>MSLTNKKNLRVVALAPTGRYFASIISSLEILETAAEFAEFQGFMTHVVTPNNRPLIGRGGISVQPTAQWQSFDFTNILIIGSIGDPLESLDKIDPALFDWIRELHLKGSKIVAIDTGIFVVAKAGLLQQNKAVMHSYFAHLFGELFPEIMLMTEQKALIDG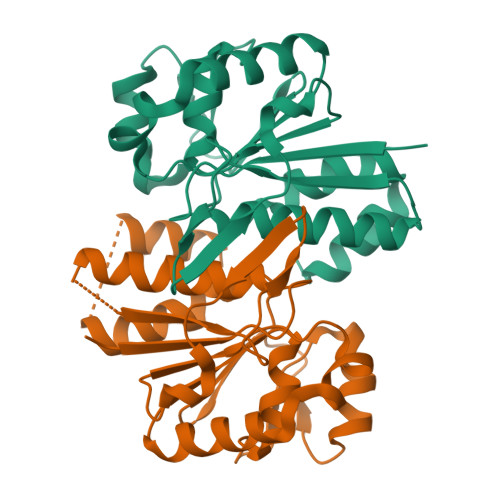NVYLSSGPYSHSSVMLEIVEEYFGKHTRNLGNQFLSTIESEGHHHHHH[6x]> MEEAELAYLLGELAYKLGEYRIAIRAYRIALKRDPNNAEAWYNLGNAYYKQGDYREAIRYYLRALKLDPENAEAWYNLGNALYKQGKYDLAIIAYQAALEEDPNNAEAK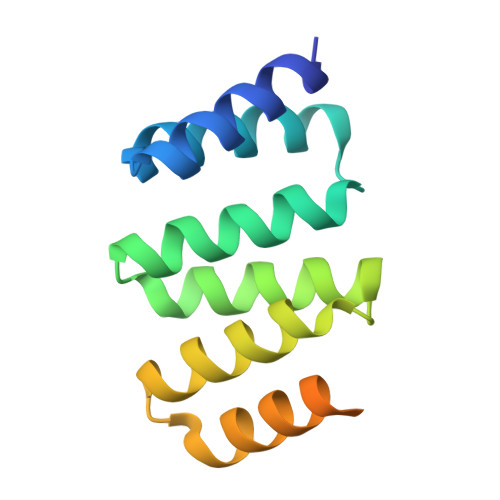QNLGNAKQKQGLEHHHHHH> GAMEEERHQVLKKWNETAHPHPEENFLQLFEKQAERIPEAIAVICEDQALSYTELNQQANRLAHFLMEYGVGPEQYVALALPRSAEMVIAMLAVLKTGAAYLPLDLDYPDERIAFMLEDTKPVCIVTSSSVQSKLSHFPSCSTIILDHPETEQAIKHYPDTNVPKTQSPLHPAYVIYTSGSTGKPKGVVVPFHSLNNFLLAMREKFALKEHDRLLAVTTIAFDISALEIFLPLISGASLVVAKKETIQDPQALAAVISDKEITIMQATPTLWHMLVTHHPDCIAGLRVLVGGEALSSGLASALHRLACEVTNLYGPTETTIWSTMSPLHPDDARAPSIGRPIWNTQVYVLDEQLQPVPPGVVGELYIAGSGLARGYLRRPDLTAERFVANPYGPPGSRMYRTGDLVRWRMDGSLDYIGRVDHQIKLRGFRIEIGEIEAVLSQCDLVERALVVAREDQPGDQRLVAYVIPCEQSKGTLDLAELRRYVSERLPDYMVPSAFMVLNEFPLTPNGKIDRKALPAPDFTMTVKGRKPRNPQEEILCELFAEVLEIPVVGIDDHFFELGGHSLLAARLISRIRDVLGVEITIGKLFASPTVASLVKHLEDAENRKPPVKAYACKEDIPLSFAQRRLWFLYHLEGPSPTYNIPVVVHLTGELHYQALQQA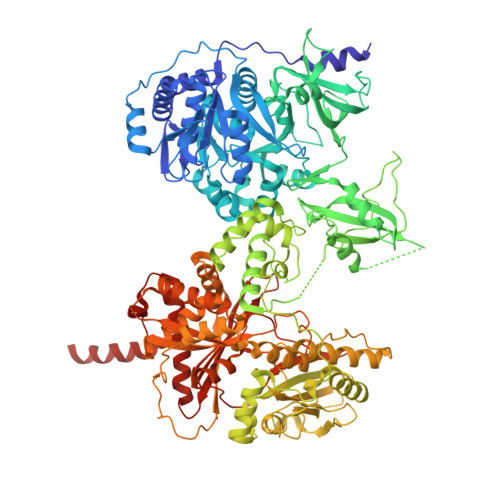LYDVIERHEPLRTIFPEHSGASRQVILEPHQARPELMIKEISESELSDELNAAVRYRFDLAAEPAIRAQLFVLGPNRHVLLLLMHHMIVDGWSLTPLTRDIAAAYNAHCRNQKVEWAPLPVKYADYALWQQEILGDETNPDSLIAKQLDYWKKTLAGLPEELELPTDYPRPAESSYEGGIVDFCMDAELHKRLLDLARENKASLFMVLQAGFAAFLTRLGAGTDIPIGSPIAGRNDDSLEHLVGLFINTLVLRMDTSGNPSFRELLGRVREVNLSAYENQDIPFERLVEILNPVRSRAKHPLFQVMFVFQNTPEPKLELQGLESRLEIRSVGTAKFDLTLELRERRGEDGSPDGLIGLFEYSRDLFDHTTVEAFAKRLCQLLREVVMNPDLPIGQIDMLLPEERKKLLAAAENLYFQ>[4x]MGLFAGKGVLVTGGGIGAIAQAFAR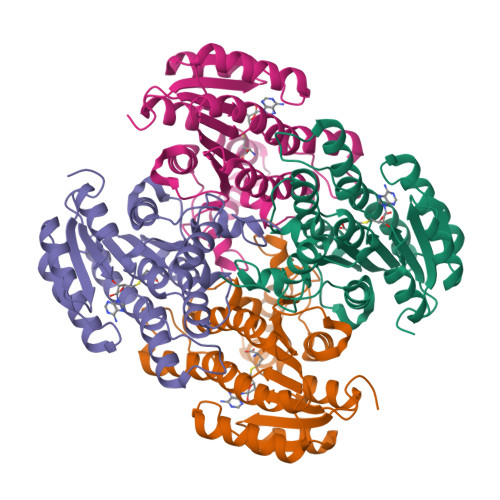EGALVALCDLRPEGKEVAEAIGGAFFQVDLEDERERVRFVEEAAYALGRVDVLVNNAAIAAPGSALTVRLPEWRRVLEVNLTAPMHLSALAAREMRKVGGGAIVNVASVQGLFAEQENAAYNASKGGLVNLTRSLALDLAPLRIRVNAVAPGAIATEAVLEAIALSPDPERTRRDWEDLHALRRLGKPEEVAEAVLFLASEKASFITGAILPVDGGMTASFMMAGRPV> NSVVVKNLDDGQA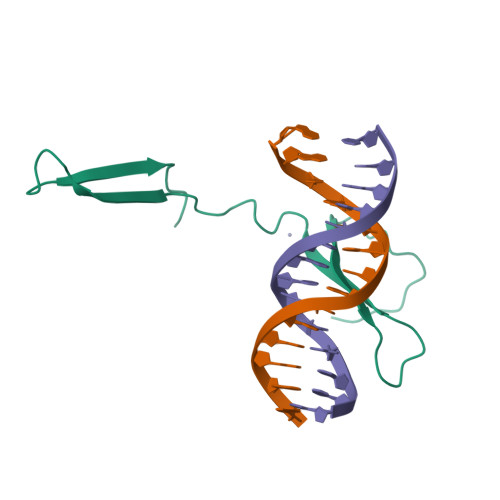WRKYGQKEIQNSKHPKAYFRCTHKYDQLCTAQRQVQRCDDDPASYRVTYIGEHTCR(1R,2R)-1,2-diphenylethane-1,2-diol 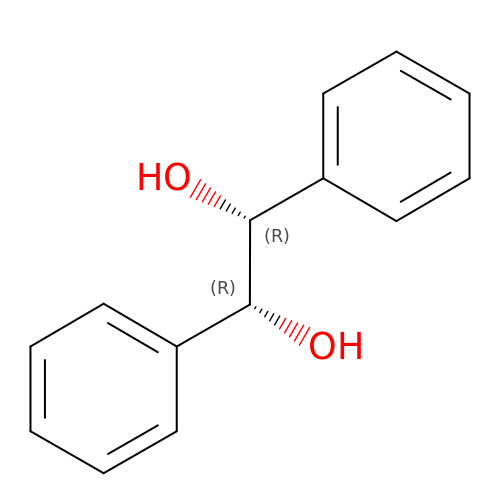| C14 H14 O2 | IHPDTPWNFBQHEB-ZIAGYGMSSA-N>GSMEAIAKYDFKATADDELSFKRGDILKVLNEECDQNWYKAELNGKDGFIPKNYIEMKPHPWFFGKIPRAKAEEMLSKQRHDGAFLIRESESAPGDFSLSVKFGNDVQHFKVLRDGAGKYFLWVVKFNSLNELV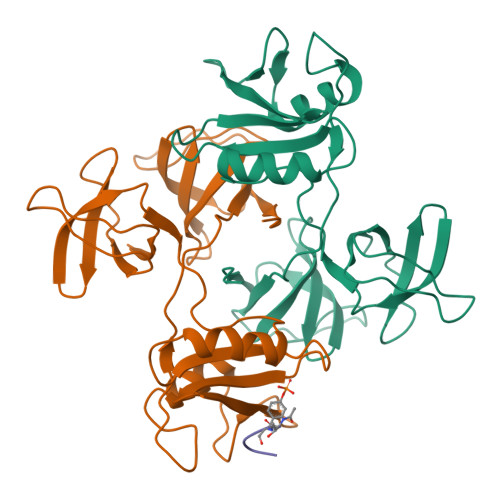DYHRSTSVSRNQQIFLRDIEQVPQQPTYVQALFDFDPQEDGELGFRRGDFIHVMDNSDPNWWKGACHGQTGMFPRNYVTPVNRNV[2x];> TYSNLGQ> MDLKAL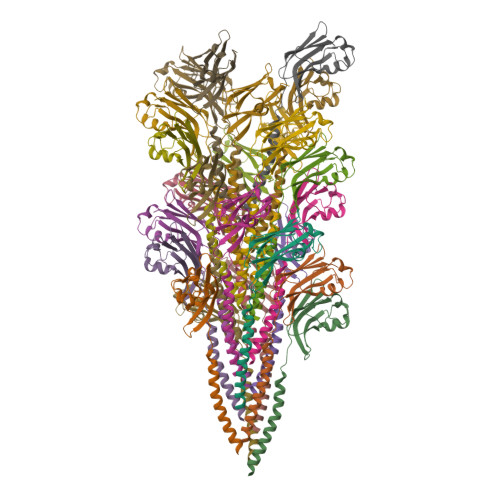KPKLVGSDNERAVSPVIGVILMVAITVILAAVIAAFVLDLGGSVGQEAQAGVTIEVDESSQEIQVEVTSMGNSDLVKLGGATDGIASNAGSTISGDHTDMQTGDVVTMDGSSWSSTSGASASGTITAIAVIEEDETETQVASEEYDFS> MKPLLSGSIPVEQFVQTLEKHGFSDIKVEDTAKGHIVLLQEAETLI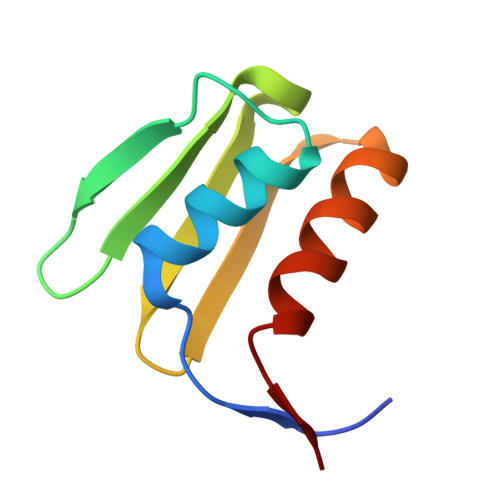QIEEDSTHIICDNDEMLRVRLRDLVLKFLQKF> M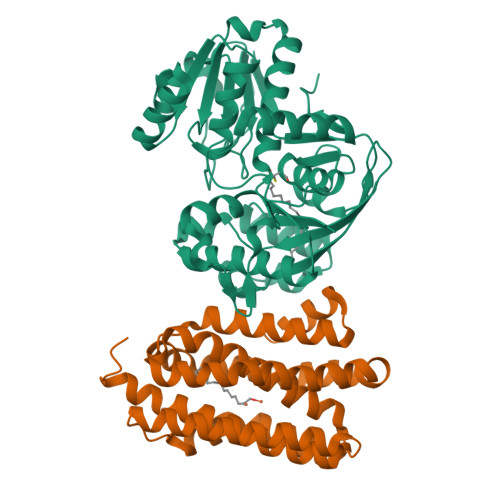FGLIGHLTSLEQARDVSRRMGYDEYADQGLEFWSSAPPQIVDEITVTSATGKVIHGRYIESCFLPEMLAARRFKTATRKVLNAMSHAQKHGIDISALGGFTSIIFENFDLASLRQVRDTTLEFERFTTGNTHTAYVICRQVEAAAKTLGIDITQATVAVVGATGDIGSAVCRWLDLKLGVGDLILTARNQERLDNLQAELGRGKILPLEAALPEADFIVWVASMPQGVVIDPATLKQPCVLIDGGYPKNLGSKVQGEGIYVLNGGVVEHCFDIDWQIMSAAEMARPERQMFACFAEAMLLEFEGWHTNFSWGRNQITIEKMEAIGEASVRHGFQPLALAI;> MRTPWDPPNPTFSLSSVSGDRRLMPQLEASLELDFQSESYKDAYSRINAIVIEGEQEAFDNYNRLAEMLPDQRDELHKLAKMEQRHMKGFMACGKNLSVTPDMGFAQKFFERLHENFKAAAAEGKVVTCLLIQSLIIECFAIAAYNIYIPVADAFARKITEGVVRDEYLHRNFGEEWLKANFDASKAELEEANRQNLPLVWLMLNEVADDARELGMERESLVEDFMIAYGEALENIGFTTREIMRMSAYGLAAV4-hydroxybenzonitrile | C7 H5 N O | 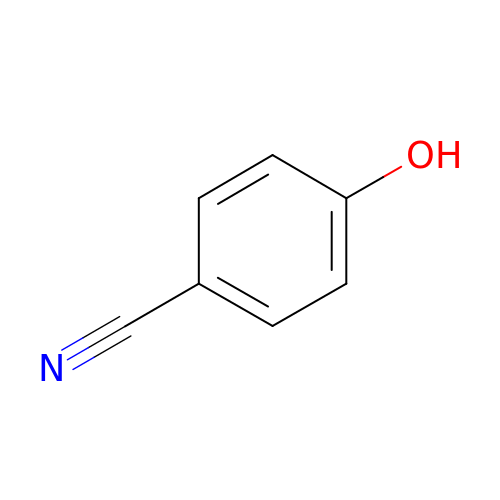CVNOWLNNPYYEOH-UHFFFAOYSA-N>DVPLTPSQFAKAKSENFDKKVILSNLNKPHALLWGPDNQIWLTERATGKILRVNPE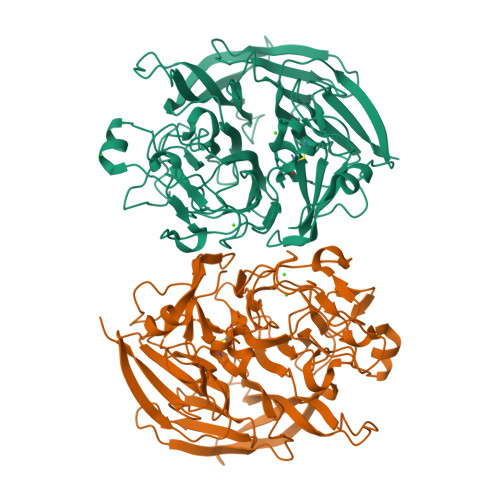SGSVKTVFQVPEIVNDADGQNGLLGFAFHPDFKNNPYIYISGTFKNPKSTDKALPNQTIIRRYTYNKSTDTLEKPVDLLAGLPSSKDHQSGRLVIGPDQKIYYTIGDQGRNQLAYLFLPNQAQHTPTQQELNGKDYHTYMGKVLRLNLDGSIPKDNPSFNGVVSHIYTLGHRNPQGLAFTPNGKLLQSEQGPNSDDEINLIVKGGNYGWPNVAGYKDDSGYAYANYSAAANKSIKDLAQNGVKVAAGVPVTKESEWTGKNFVPPLKTLYTVQDTYNYNDPTCGEMTYICWPTVAPSSAYVYKGGKKAITGWENTLLVPSLKRGVIFRIKLDPTYSTTYDDAVPMFKSNNRYRDVIASPDGNVLYVLTDTAGNVQKDDGSVTNTLENPGSLIKFTYKA[2x]> LADQQDLTRQVPAEVESLDPAHIESWTGNTIGLDLFEGLARIDASGAVVPGVAQAWEHKAPDTWIFKLRRDAKWSNGQPVTAADFVYAWQRLADPKTGSKYTILVEFVKNASAIIAGKQPPGDLGIRAIDPYTIEVKTEVPVSYFPELTAMAP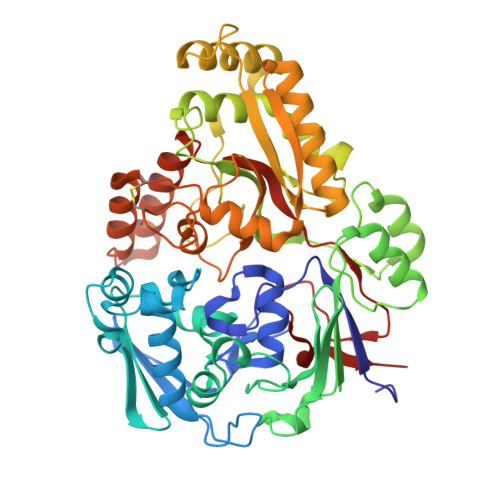LTPVNKDAVAKFGDAWTRPKNIVSNGPYTLVDWQPNNRIVMAKSDKYWNARNVVIRKVTYLPIENDETALRMYQAGQIDYTYSIPAGGFGQISKQFGKELRPGLQLATYYYYLKNSDPALKDKRVREALAMVLDREILTSKITQAGEVPMYGLMPKGVKGVQRPFTPDWASWPMARRVDYAKNLLKQAGHGDANPLTFTLTYNTNDLHKKVALFAASEWRTKLGVTAKLENVEFKVLMKQRHDGKVQIARDGWFADYNDAMTFFDLIRCGSSQNTVGYCNPKVDSLVAEANQKLDDGARAALLTQAHDLAMNDYPMVPLFQYSADRLVKSYVGGYTLTNYIDMRASQDMYLIK> GSEANSYDSDQATTLGALEFSLLYDQDNSNLQCTIIRAKGLKPMDSNGLADPYVKLHLLPGASKSNKLRTKTLRNTRNPVWNETLQYHGITEEDMQRKTLRISVCDEDKFGHNEFIGETRFSLKKLKANQRKNFN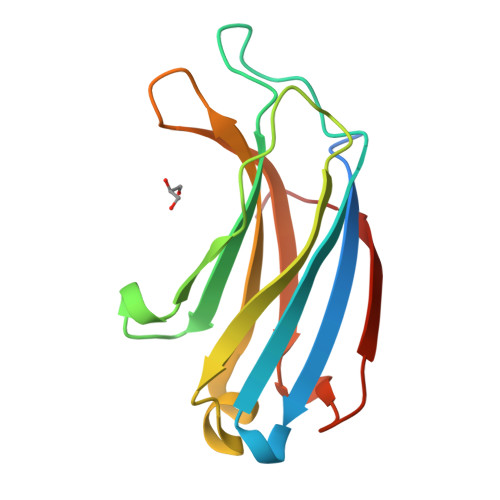ICLERVI> MSGFHNVGNINMMAQQQMQQNRIKISVRNWQNATMNDLINFISRNARVAVYDAHVEGPLVIGYVNSKAEAESLMKWNGVRFAGSNLKFELLDNNGASAGTSDTISFLRGVLLKRYDPQTKLLNLGALHSDPELIQKGVFSSISTQSKMFPAMMKLASTEKSLIVESVNLADNQLKDISAISTLAQTFPNLKNLCLANNQIFRFRSLEVWKNKFKDLRELLMTNNPITTDKLYRTEMLRLFPKLVVLDNVIVRDEQKLQTVYSLPMKIQQFFFENDALGQSSTDFATNFLNLWDNNREQLLNLYSPQSQFSVSVDSTIPPSTVTDSDQTPAFGYYMSSSRNISKVSSEKSIQQRLSIGQESINSIFKTLPKTKHHLQEQPNEYSMETISYPQINGFVITLHGFFEETGKPELESNKKTGKNNYQKNRRYNHGYNSTSNNKLSKKSFDRTWVIVPMNNSVIIASDLLTVRAYSTGAWKTASIAIAQPPQQQASVLPQVASMNPNITTPPQPQPSVVPGGMSIPGAPQGAMVMAPTLQLPPDVQSRLNPVQLELLNKLHLETKLNAEYTFMLAEQSNWNYEVAIKGFQSSMNGIPREAFVQF;>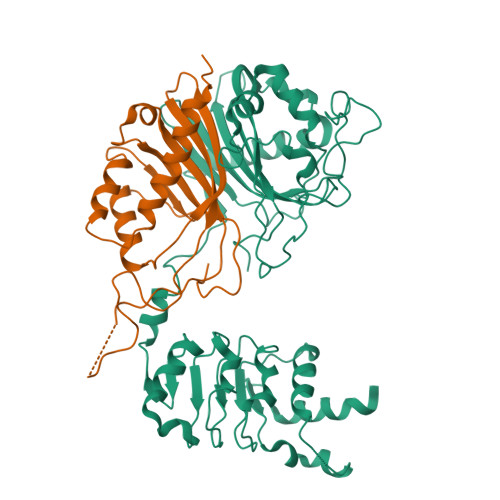 MNTNSNTMVMNDANQAQITATFTKKILAHLDDPDSNKLAQFVQLFNPNNCRIIFNATPFAQATVFLQMWQNQVVQTQHALTGVDYHAIPGSGTLICNVNCKVRFDESGRDKMGQDATVPIQPNNTGNRNRPNDMNKPRPLWGPYFGISLQLIIDDRIFRNDFNGVISGFNYNMVYKPEDSLLKI>[4x]GGTESGLEHCVKIIRQLECSGHIDKNFAQDFLTWYSLRATSQEIRVVKDFIDTFI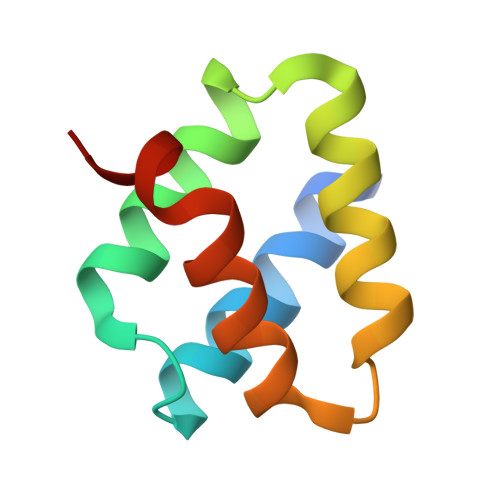DDPMALAEQLIDTFDDRVSIKR>FDCGKPQVEPKKCPGRVVGGCVAHPHSWPWQVSLRTRFGQHFCGGTLISPEWVLTAAHCLEKSPRPSSYKVILGAHQEVNLEPHVQEIEVSRLFLEPTRKDIALLKLSSPAVITDKVIPACLPSPNYMVADRTECFITGWGETQGTFGAGLLKE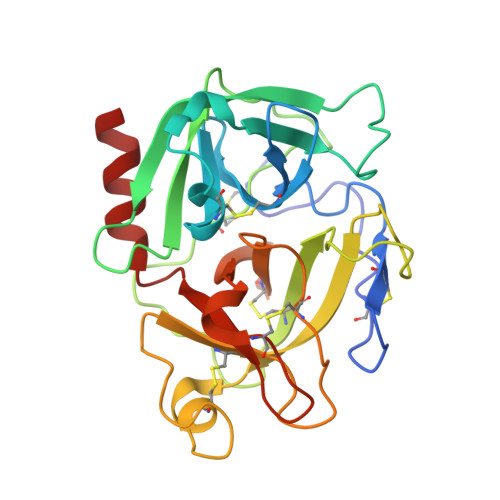AQLPVIENKVCNRYEFLNGRVQSTELCAGHLAGGTDSCQGDSGGPLVCFEKDKYILQGVTSWGLGCARPNKPGVYVRVSRFVTWIEGVLRNN[4x]>[22x]MVVQHNLTAMNANRQLGITTGAQAKSSEKLSSGYKINRAADDAAGLTISEKMRSQVRGLNKASDNAQD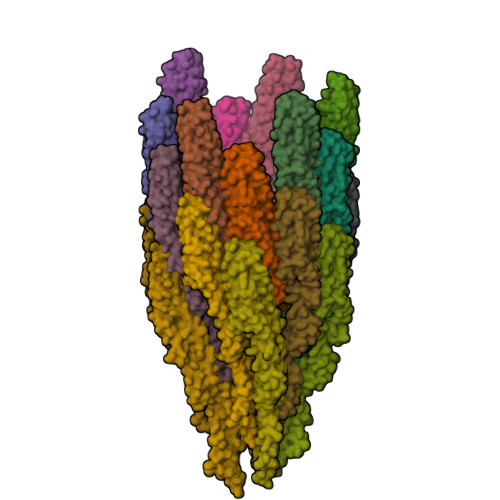GVSLIQVAEGALSETHSILQRMNELATQAANDTNTTSDRTAVQQEINQLASEITRIASTTQFNTMNLIDGNFTSKKLQVGSLCGQAITIDISDMSATGLGVSGLVVSSFSAAGKAMSAAQDAISYVSSMRSKLGALQNRLEHTISNLDNISENTSSAESRIRDTDMAEEMVEYSKNNILAQAGQSMLAQANQSTQGVLSLLQ> S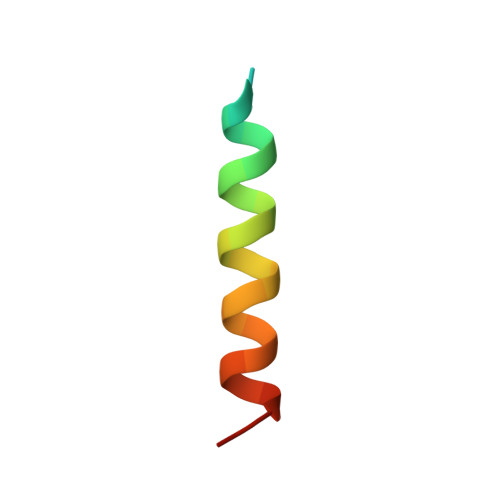ADERQRMLVQRKDELLQQARKRFLNKS> LADRFAELERRYDARLGVYVPATGTTAAIEYRADERFAFCSTFKAPLVAAVLHQNPLTHLDKLITYTSDDIRSRSPVAQQHVQTGMTIGQLCDAAIRYSDGTAANLLLADLGGPGGGTAAFTGYLRSLGDTVSRLDAEEPELNRDPPGDERDTTTPHAIALVLQQLVLGNALPPDKRALLTDWMARNTTGAKRIRAGFPADWKVIDKTGTGDYGRANDIAVVWSPTGVPYVVAVMSDRAGGGYDAEPREALLAEAATCVAGVLA

pmcAntibiotic resistance mediated by β-lactamase-producing bacteria has become one of the major threats to global health. This phenomenon has substantially reduced the efficacy of β-lactam drugs, which are the most commonly prescribed antibiotics worldwide. β-Lactamases (EC.3.5.2.6) are a group of enzymes that can hydrolyze the amide bond of the β-lactam ring, thus making the antibiotics inactive. One such residue, at position 105 (standard Ambler numbering), is suggested to play an important role in substrate discrimination of class A enzymes. Interestingly, BlaC, the β-lactamase from Mycobacterium tuberculosis, possesses Ile at this position, sparking the question about the evolutionary preference for this amino acid. Mutation of Ile105 to Arg in the β-lactamase BlaC simultaneously enhances activity for carbenicillin and the ability to evade clavulanic acid inhibition.

Unlike clavulanic acid, avibactam is a reversible covalent inhibitor and does not display secondary chemistry upon binding. Short soaking (∼10 min) did not reveal any detectable density for either of the inhibitors. In the crystal structure of the I105R variant in the complex with avibactam, the sulfate moiety of the carbamyl adduct of avibactam occupies the carboxylate binding pocket and engages in H-bonding with Ser130, Thr235, and Thr237. The electron density of the Arg105 side chain was missing, indicating elevated dynamics of this residue upon binding. The avibactam-bound structure showed an inward-oriented sulfate moiety of the carbamyl adduct, which is likely engaged in H-bonding with Ser130, Thr235, and Thr237. In all instances, this is speculated to be a stable inactive conformation of the inhibitor, which is substantially more resistant to hydrolysis than clavulanic acid. BlaC I105R is less sensitive to clavulanic acid and avibactam inhibition, although the effect is more prominent for the former inhibitor. The beneficial fitness of BlaC I105R correlates with an 8- and 4-fold increase in MIC values for clavulanic acid and avibactam, respectively.> DEE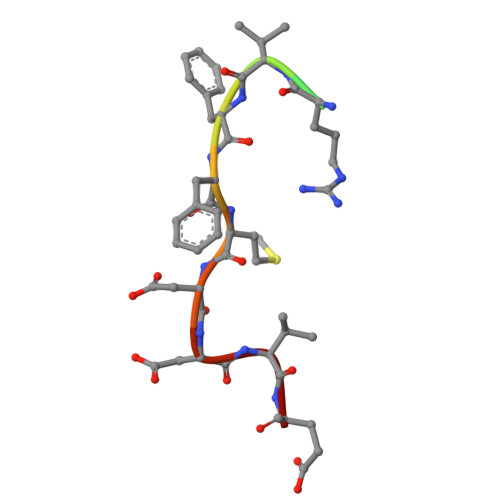ERVFFMDDVE> MKVVYDDVRVLKDIIQALARLVDEAVLKFKQDSVELVALDRAHISLISVNLPREMFKE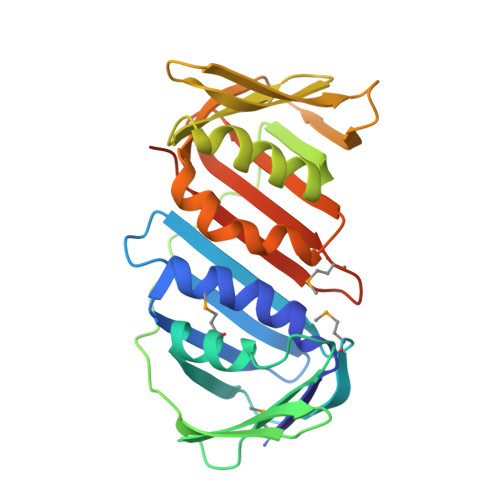YDVNDEFKFGFNTQYLMKILKVAKRKEAIEIASESPDSVIINIIGSTNREFNVRNLEVSEQEIPEINLQFDISATISSDGFKSAISEVSTVTDNVVVEGHEDRILIKAEGESEVEVEFSKDTGGLQDLEFSKESKNSYSAEYLDDVLSLTKLSDYVKISFGNQKPLQLFFNMEGGGKVTYLLAPKVLEHHHHHH> SRMQLSEEQAAVLRAVLKGQSIFFTGSAGTGKSYLLKRILGSLPPTGTVATASTGVAACHIGGTTLHAFAGIGSGQAPLAQCVALAQRPGVRQGWLNCQRLVIDEISMVEADLFDKLEAVARAVRQQNKPFGGIQLIICGDFLQLPPVTKGSQPPRFCFQSKSWKRCVPVTLELTKVWRQADQTFISLLQAVRLGRCSDEVTRQLQATASHKVGRDGIVATRLCTHQDDVALTNERRLQELPGKVHRFEAMDSNPELASTLDAQCPVSQLLQLKLGAQVMLVKNLSVSRGLVNGARGVVVGFEAEGRGLPQVRFLCGVTEVIHADRWTVQATGGQLLSRQQLPLQLAWAMSIHKSQGMTLDCVEISLGRVFASGQAYVALSRARSLQGLRVLDFDPMAVRCDPRVLHFYATLRRGRSLSLESPDDDEAASDQENMDPIL

Pif1 is a multifunctional helicase and DNA processing enzyme that has roles in genome stability. Pif1 proteins are monomeric enzymes and members of helicase superfamily 1 (SF1), while the 5′–3′ polarity of unwinding place them in the SF1B subgroup. The hPIF1 helicase has the domain architecture characteristic of the SF1B RecD2 helicase subgroup. The overall organization of these domains is similar in all nucleotide bound and free structures determined. hPIF1 has three structural domains, two RecA-like domains 1A (residues 206–381, blue in Figure 1) and 2A (residues 382–435) and domain 2B (residues 436–548, green in Figure 1) with a SRC Homology 3 (SH3)-like fold, in addition to the small functional domain 1B within domain 1A (residues 280–300, cyan in Figure 1).

The structures we report are of constructs from residues 206–641 (apo hPIF1) or 206–620 (the structures with nucleotide analogues bound). In the 1.44 Å apo-hPIF1 crystal structure residues after 620 are not seen in the electron density suggesting they are disordered. SUL1 is stabilized by hydrogen bonds with the main chain atoms of the loop residues from the Walker A motif and the side chain of the Walker A K234 residue at the beginning of the α2 helix, situated at the 1A–2A inter-domain contact area. Tight packing of this area is maintained by interaction of the inter-domain linker R381 (motif IV) with the carboxyl group of Q206 at the N-terminal part of the 1A domain. A second arginine, R584 (motif VI), interacts with S557 (motif V) and the carboxyl group of I554, contributing to the rigidity of the inter-domain 2A–2B contact area. We also mutated K485, N486 and N495 of the poorly characterised B (residues 477–486) and C (residues 494–499) motifs within domain 2B that are characteristic of the SF1B RecD helicases sub-family. K485, N486 and N495 are in exposed loops where a sulphate ion is located in the apo-hPIF1 structure (SUL2 in Figure 1B). Residue K414 was also selected for analysis and we also included the E307Q Walker B motif variant as a control. K414 is also in the vicinity of a bound sulphate (SUL3 in Figure 1B) and is conserved between mammalian and bacterial Pif1, but it is not in the ssDNA binding channel revealed in Bs and ScPif1 structures. However, a comparison of our 1.13 Å AMP-PNP structure with our 1.44 Å apo structure shows that the binding of the nucleotide induces movement of the Walker A motif (residues 228GSAGTGKS235).> GSHMPKYNVRDKKALLRLLDQHDQRGLGGILLEDIEEALPNSQKAVKALGDQILFVNRPDKKKILFFNDKSCQFSVDEEFQKLWRSVTVDSMDEEKIEEYLK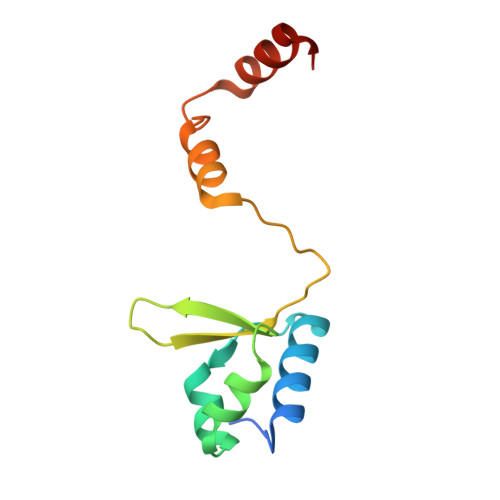RQGISS(2Z)-2-hydroxy-4-[4-(octyloxy)phenyl]-4-oxobut-2-enoic 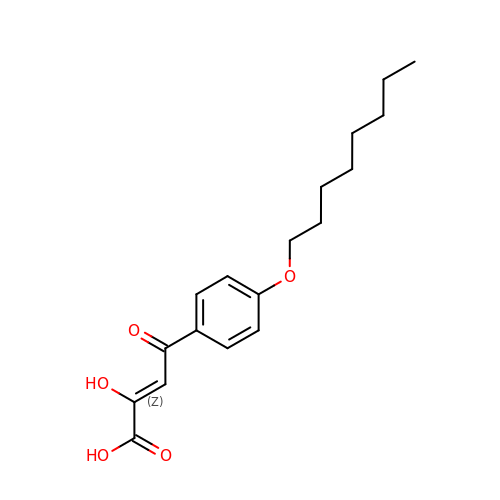acid | C18 H24 O5 | LOLDLWKHRAJWHI-LGMDPLHJSA-N> SMLHTTQIRMVGTGSAFSKKFYNNSALVTFTNGYNLLIDCGHSVPKGLHDADIPLESIDGILITHTHADHIGGLEEVALYNKFVLGGRKIDLLVPNTLVESLWENSLKGGLRYSDTYDDLSLSDYFTVRSLKTFTSGAARTQLEENIAIKLYPTFHVSHMASYAVGLEDRGEDKVFYSSDTIFDEYLIDYALTYSWVFHDCQFFTGGVHASLDELLNYIPEEDQDRVFLMHYGDNMEDFFTKTGRMRFALQGRTYIL

The cyclic oligonucleotide-based antiphage signalling system (CBASS) and the pyrimidine cyclase system for antiphage resistance (Pycsar) are antiphage defence systems in diverse bacteria that use cyclic nucleotide signals to induce cell death and prevent viral propagation. Here we show that phages encode anti-CBASS (Acb) and anti-Pycsar (Apyc) proteins that counteract defence by specifically degrading cyclic nucleotide signals that activate host immunity. Using a biochemical screen of 57 phages in Escherichia coli and Bacillus subtilis, we discover Acb1 from phage T4 and Apyc1 from phage SBSphiJ as founding members of distinct families of immune evasion proteins. We confirmed the critical role for Apyc1 metal-coordinating residues and identified E74 and Y112 from the opposing protomer as further catalytic residues required for cCMP hydrolysis and release of the reaction product 5′-CMP. Together, these findings demonstrate that Acb1 and Apyc1 constitute separate families of immune evasion proteins and explain the distinct reaction mechanisms that degrade CBASS or Pycsar cyclic nucleotide signals.

To compare mechanisms of anti-CBASS and anti-Pycsar evasion, we determined the crystal structure of Apyc1 from the phage Bsp38 (2.7 Å) as well as structures of Paenibacillus Apyc1 proteins (1.5 Å and 1.8 Å). Structures of Apyc1 reveal a metal-dependent cyclic NMP phosphodiesterase that uses relaxed specificity to target Pycsar cyclic pyrimidine mononucleotide signals. Structural comparison of Apyc1 and B. subtilis YhfI also reveals that Apyc1 enzymes contain an extended loop that reaches into the nucleotide-binding pocket, potentially enabling stable binding of smaller cyclic pyrimidine substrates. Recombinant protein produced from gene 147 rapidly degrades the Pycsar signals cCMP and cUMP, and we named this anti-Pycsar protein Apyc1 (European Nucleotide Archive genome accession number ERS1981056). SBSphiJ Apyc1 efficiently hydrolyses a wide range of cyclic mononucleotides, exhibiting an atypically relaxed nucleobase specificity that enables targeting of cyclic pyrimidine signals used in Pycsar immunity. By contrast, the closely related B. subtilis enzymes YhfI (GenBank accession number NP_388905.1) and MBL phosphodiesterase (GenBank accession number WP_013351727.1) exhibited a strong preference for cAMP/cGMP over cCMP/cUMP cleavage, confirming that relaxed nucleotide specificity and Pycsar signal degradation are unique to Apyc1 and not general features of MBL phosphodiesterase enzymes.> MTVQTSKNPQVDIAEDNAFFPSEYSLSQYTSPVSDLDGVDYPKPYRGKHKILVIAADERYLPTDNGKLFSTGNHPIETLLPLYHLHAAGFEFEVATISGLMTKFEYWAMPQKDEKVMPFFEQHKSLFRNPKKLADVVASLNADSEYAAIFVPGGHGALIGLPESQDVAAALQWAIKNDRFVISLDH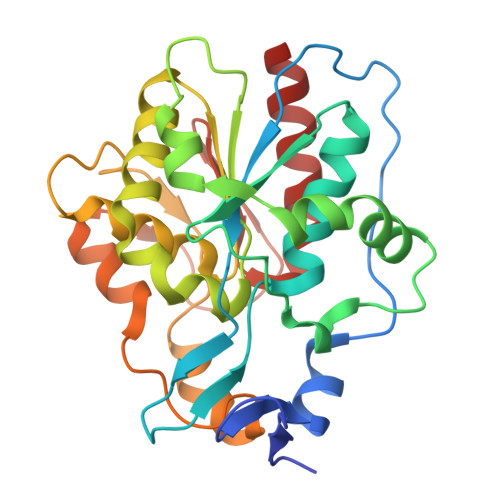GPAAFLALRHGDNPLNGYSICAFPDAADKQTPEIGYMPGHLTWYFGEELKKMGMNIINDDITGRVHKDRKLLTGDSPFAANALGKLAAQEMLAAYAG> GAASMGPGRQVGDRSYYIGLLRPKITELTTEIERLNEQEELIVKGGSVLTQLQQRNKALTDEAAKLKGTLADINLALEKSTTQDPSSVKDQATKLNQVNGEKRKQVDQLFLNAKEMEALTKKNTQALEEEMQNLDRRILAENQDFGLYKATRDEAFNVSDAVLSHQHQIRMLTAKQELLMTKLSTDPDKKRAAEVLRGILSKRQLKEELTKQ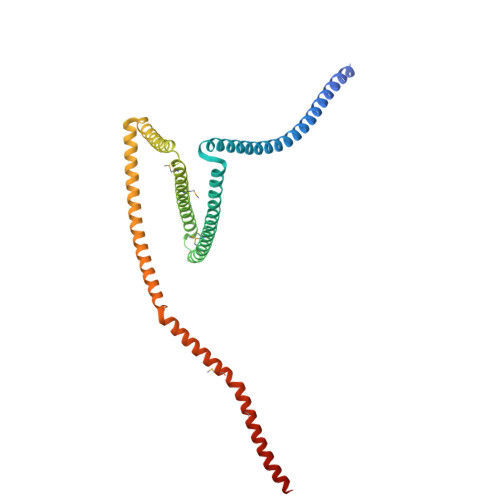CALSVEEERQLLIKQVKTARGDIEVLERQVNETRDALSESKNRCASLDEELKSYSGDNIKAFQELQEKDRELQSFMDSFPAKLKEEMDKITEVQRNIATLLERISQALELKKQMPQ>MGSSHHHHHHSSGLVPRGSSDRPEDAIAIVGMSGRYPGARNVREYWDNLVHARNAIRDIPTSRWDVDKYYDPVLNKKGKVYCKSMGMLDDIEHFDPLFFNIPPSEAELMDPQHRIFLQEGYKAFEDAGYNARTLNEKKCGVYLGIMSNEYGVMLNRQSRANATGNSFAIAAARIPYFLNLKGPAIPIDTASSSSLVGTHLARQALINKEIDMALVGGVSLYLTPESYMSMCEAGMLSPDGQCKAFDNGANGFVPGEGAGALVLKRLKDAEADRDHIYGIIIGSGINQDGKTNGITAPSAKSQMDLERDIYETYGIHPESISYVEMHGTGTKQGDPIELEALSTVFQEKTDKKQFCAIGSVKSNIGHTSA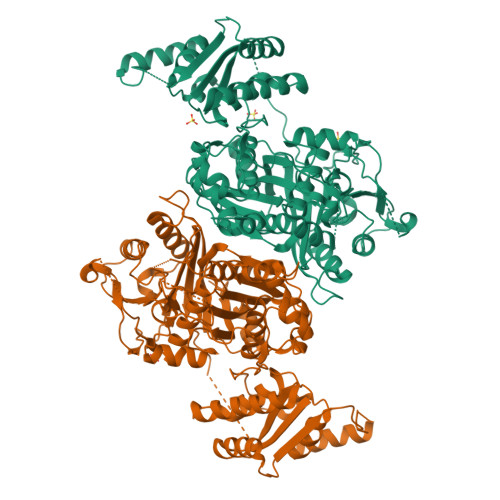AAGVAGVQKVLLCMNHKTLVPTLNFTTPNEHFEFEHSPLYVNTELKPWETADGKPRRACVSSFGYSGTNAHIVIEEYQPEKRNDRLTKQHRSALFVLSAKKEKQLKAYAEAMKDFVTSNEDIDLEDMAYTLQTGREAMDYRMAFLADSREMLIKALDDYLAEMPNGSIFAAHVKTKKSEIKLFETDHDAKALLQTWIEKKRLEKVAELWVKGLQIDWNKLYGEYTPRRISLPAYPFAEEYYWLPTQEG[2x]>[2x]MSLTNQTYKIGLVLKGSEEPIRLNPFYINVLLGISETCNQHGYGTQTTVSNNMNDLMDEVYKMIK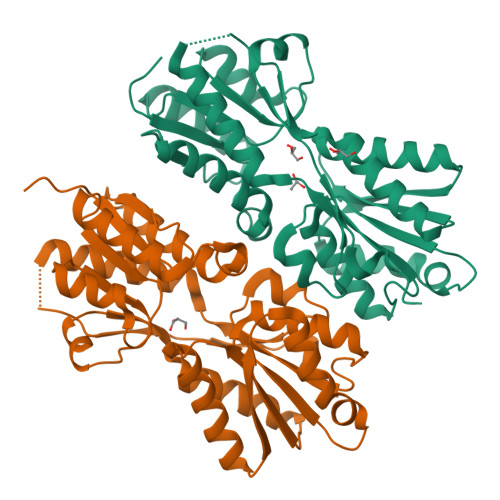QRMVDAFILLYSKENDPIKQMLIDESMPFIVIGKPTSDIDHQFTHIDNDNILASENLTRHVIEQGVDELIFITEKGNFEVSKDRIQGFETVASQFNLDYQIIETSNEREVILNYMQNLHTRLKDPNIKQAIISLDAMLHLAILSVLYELNIEIPKDVMTATFNDSYLTEIASPPQTCIDIKPRMLGQQAGSAILNILKNKAQDVIELVIIDTELKIRKSTQREGHHHHHH>[2x]GSEFELMTHSVSPIGYIRSC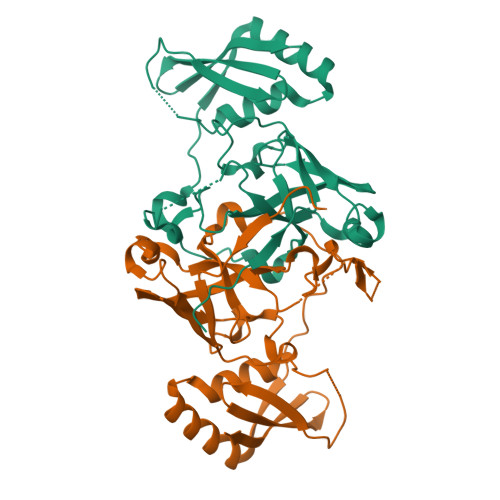FMEKFAIPRQPLLAPAARGTLELLPPFDQVEALEGLEQVSHVWLLFLFHQALEDKPRLKVRPPRLGGNRSLGVFATRATHRPNGIGQSVVRLEGFEAGRLWLSGIDLLDGTPVLDIKPYVPYADAVADARNGIADAPPPGIAVEWSEQARRQAHEHGQRLRQPVAELIEQCLAQDPRPAYQKPEPGRRYGVRLWDLDVHWHYPRPDLIRVLDVAGGD>MGRFVVWPSELDSRLSRKYGRIVPRSIAVESPRVEEIVRAAEELKFKVIRVEEDKLNPRLSGIDEELRTFGMIVLESPYGKSKSLKLIAQKIREF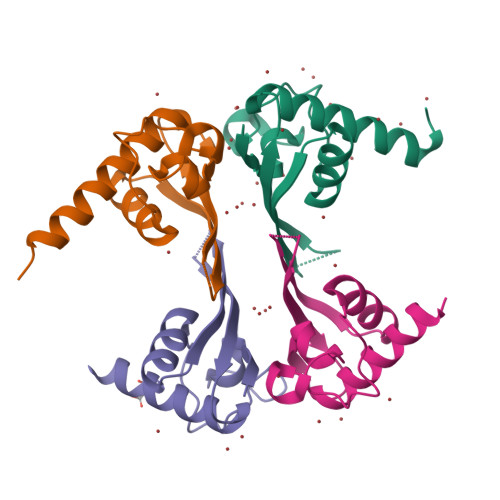RRRSAGTLVPR[4x]> IESIIKTATDTVKSEINAELGVVPSLNAVETGASSNTEPEEAIQTRTVINQHGVSETLVENFLSRAALVSKRSFEYKNHTSSEARTDKNFYKWTINTKSFVQLRRKLELFTYLRFDAEITILTTVAVGSNNSTYMGLPDLTLQAMFVPTGAL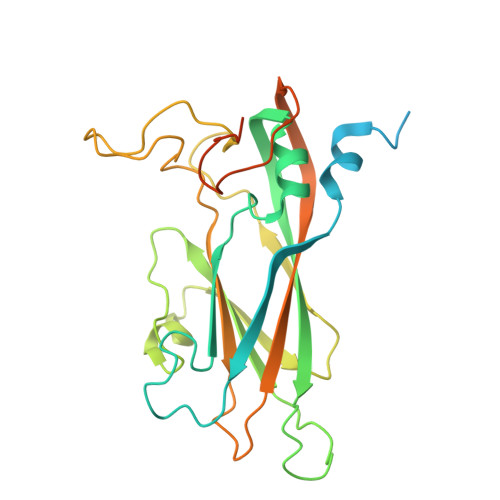TPEKQDSFHWQSGSNASVFFKVSDPPARMTIPFMCINSAYSVFYDGFAGFEKNGLYGINPADTIGNLCVRIVNEHQPIGFTVTVRVYMKPKHIKAWAPRPPRTLPYMSIANANYKGKERAPNALNAIIGNRESVKTMPHDIRLV> MGSSHHHHHHGSMYGVYRAMKLPIYLDYSATTPVDPRVAEKMMQFMTMDGTFGNPASRSHRFGWQAEEAVDIARNQIADLVGADPREIVFTSGATESDNLAIKGAANFYQKKGKHIITSKTEHKAVLDTCRQLEREGFEVTYLAPQRNGIIDLKELEAAMRDDTILVSIMHVNNEIGVVQDIAAIGEMCRARGIIYHVDATQSVGKLPIDLSQLKVDLMSFSGHKIYGPKGIGALYVRRKPRVRIEAQMHGGGHERGMRSGTLPVHQIVGMGEAYRIAKEEMATEMERLRGLRNRLWNGIKDIEEVYLNGDLEHGAPNILNVSFNYVEGESLIMALKDLAVSSGSACTSASLEPSYVLRALGLNDELAHSSIRFSLGRFTTEEEIDYTIELVRKSIGRLRDLSPLWEMYKQGVDLNSIEWAHH;> GSTDLFSSPDHTLDALGLRCPEPVMMVRKTVRNMQPGETLLIIADDPATTRDIPGFCTFMEHELVAKETDGLPYRYLIRKGG

The cysteine desulfurase IscS is a highly conserved master enzyme initiating sulfur transfer via persulfide to a range of acceptor proteins involved in Fe-S cluster assembly, tRNA modifications, and sulfur-containing cofactor biosynthesis. IscS is a highly conserved, widely distributed pyridoxal-5′-phosphate (PLP)-dependent enzyme, with 60% sequence identity between the enzyme from Escherichia coli and its human homolog, NFS1. It initiates intracellular sulfur trafficking, delivering the sulfur to several sulfur-accepting proteins such as IscU, ThiI, TusA, and MoaD/MoeB that commit the sulfur to different metabolic pathways, including iron-sulfur cluster assembly, thiamine and biotin synthesis, tRNA modifications, or molybdopterin biosynthesis. The small domain (residues 1–15 and 264–404) contains the critical active site cysteine Cys328.

The IscS-TusA complex crystallized in two forms with identical heterotetramers consisting of an IscS dimer and two TusA molecules. The distance between the two TusA monomers exceeds 40 Å. TusA interacts with the large domain of one IscS subunit within the dimer, with the exception of the tip of the loop containing the essential Cys328 of IscS, which comes from the other subunit. This persulfide-carrying Cys328IscS is juxtaposed against the acceptor cysteine of TusA, Cys19TusA, with only ∼4 Å separating their S atoms. The residues of TusA contacting IscS are located on two α-helices (α1TusA and α2TusA), which are nearly perpendicular to helix α2IscS. The interface involves van der Waals contacts, polar and hydrogen bond interactions, and salt bridges. IscS mutations that abrogated interaction with wild-type TusA, W45IscSR, E49IscSA, D52IscSR, D52IscSY, and D52IscSM (unpublished data) involved tightly clustered residues located on the side of helix α2IscS, in excellent agreement with the crystal structure. In the IscS-TusA complex, the observed proximity of Cys19TusA to persulfated Cys328IscS could be sufficient for sulfur transfer to occur. Asp51TusA is on the surface while Asp45TusA is buried but forms a hydrogen bond to the NH of Cys19TusA. As a result, the thiol groups of Cys328′IscS and Cys19TusA are in close proximity, within a distance of less than 4.5 Å. This organization of the IscS-TusA complex suggests that the dimerization of IscS is essential for effecting sulfur transfer to various acceptor proteins.> QQKPVVKTAQNLAEVNGPETLIGPGAKEGTVPTDLDQETGLARLELLGKLEGIDVFDTKPLDSSRKGTMKDPIIIESYDDYRYVGCTGSPAGSHTIMWLKPTVNEVARCWECGSVYKLNPV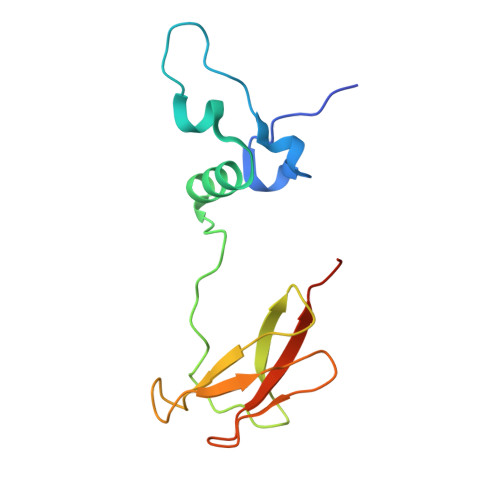GVPNDDHHH>[6x]AAPSFDCGKPQVEPKKCPGRVVGGCVAHPHSWPWQVSLRTRFGMHFCGGTLISPEWVLTAAHCLEKSPRPSSYKVILGAHQEVNLEPHVQEIEVSRLFLEPTRKDIALLKLSSPAVITDKVIPACLPSPNYVVADRTECFITGWGETQGTFGAGLLKEAQLPVIENKVCNRYEFLNGRVQSTELCAGHLAGGTDSCQGDSGGPLVCFEKDKYILQGVTSWGLGCARPNKPGVYVRVSRFVTWIEGVMRNN

The trypsin‐like serine protease plasmin catalyzes the degradation of fibrin clots into soluble fragments, thereby maintaining a normal blood flow in the circulation. Intravascular plasmin is formed from its zymogen plasminogen after activation by tissue‐type plasminogen activator (tPA), whereas extravascular plasmin, which contributes to tissue remodeling and cell migration, is mainly produced by the urokinase‐type plasminogen activator (uPA), especially when bound to its receptor uPAR leading to an enhanced uPA activity. Under physiological conditions, the activity of plasmin is tightly controlled by endogenous inhibitors, the serpin α2‐antiplasmin and by α2‐macroglobulin. Two series of macrocyclic inhibitors addressing the S1 pocket and the prime site of the fibrinolytic serine protease plasmin have been developed.

For inhibitor 28, a crystal structure in complex with a stabilized Ser195(741)Ala mutant of μ–plasmin was determined. In this structure, six monomer complexes (namely A–F) were found per asymmetric unit. The P1 and P1’ residues are identically placed in all complexes. In three complexes (A, C, and D), the macrocycle (shown with carbon atoms in different green colors) adopts a similar structure indicating a preferred inhibitor conformation. In the three other complexes (B, E, and F), the P2’ residue and the adjacent linker are placed differently. The carbonyl oxygen of the Txa group makes H‐bonds to the amide NH of Gly193(739) and Ala195(741), which form the oxyanion hole. The P1 amino group is involved in a complex H‐bond network at the bottom of the S1 pocket to plasmin residues Asp189(735) and Ser190(736), and via three bridging water molecules also to residues Trp215(761), Leu 217(763), Gly219(764), and Val227(773). However, the biphenyl side chain of the Bpa residue occupies very well the relatively long S1’ cleft between His57(603), Glu60(606), and Lys61(607) on the left side, as well as Phe41(587) on the right flank. The phenyl ring of the latter residue makes face‐to‐face contact with the terminal ring of the P1’ Bpa residue (closest C−C‐distance 3.7 Å), whereas an edge‐to‐face interaction is found between the other Bpa ring and the side chain of His57(603).>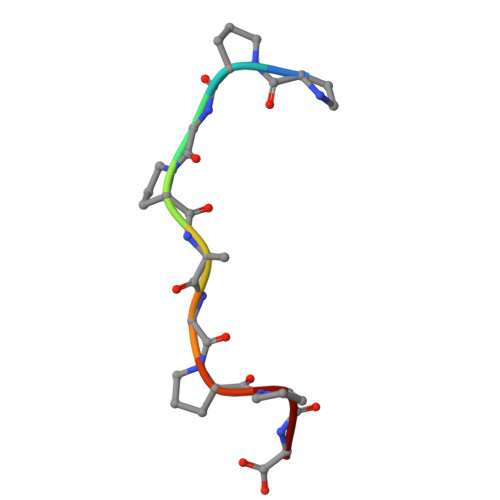 PPGPAGPPG>[6x]VASLYQAVSLKQEASLFLVGERLNATGSKRFREMLFARDLEGILALAREQVEEGAHALDLSVAWTGRDELEDLRWLLPHLATALTVPVMVDSTSPEAMELALKYLPGRVLLNSANLEDGLERFDRVASLAKAHGAALVVLAIDEKGMAKTREEKVRVALRMYERLTEHHGLRPEDLLFDLLTFPITQGDEESRPLAKETLLAMEELRERLPGVGFVLGVSNVSFGLKPRARRVLNSV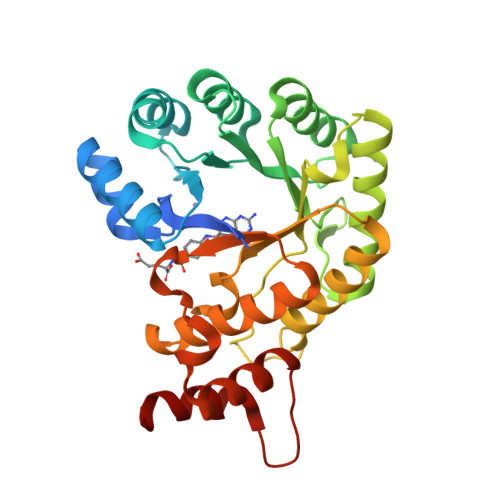FLDEARKRGLTAAIVDAGKILPISQIPEEAYALALDLIYDRRKEGFDPLLAFMAYFEAH> MKNFVIGSGVISLRYKNGVITCTDTQASYGNLCKFNDVRRIFRLSSNTLISLSGEISDIQFLMNELNKLNESDPVKMSPRGYLNLVQGILYNKRSRVEPLNVSVSIVGVDDDDFLVSCVNHLGNFYEDNIVCTGLSNMIALPFLRTCNVLDLERDEA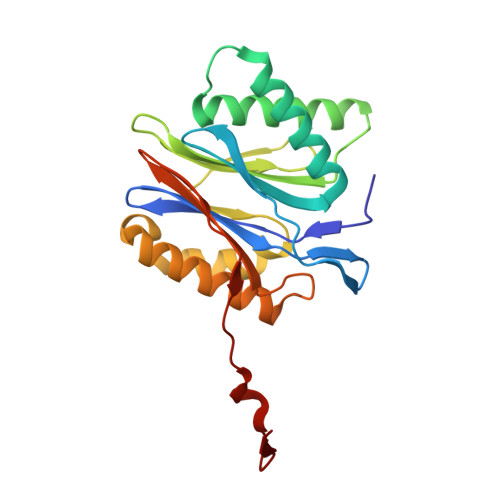ISLVEKAMTVMCYRSCRSSNRIQIGVVEKGLVDISDPYVLNTDWQVGHNEEEIVL>[2x]PAWTTFRVGLFCGIFIVLNITLVLAAVFKLETDRSIWPLIRIYRGGFLLIEFLFLLGINTYGWRQAGVNHVLIFELNPRSNLSHQHLFEIAGFLGILWCLSLLACFFAPISVIPTYVYPLALYGFMVFFLINPTKTFYYKSRFWLLKLLFRVFTAPFHKVGFADFWLADQLNSLSVILMDLEYMICFYSLELKW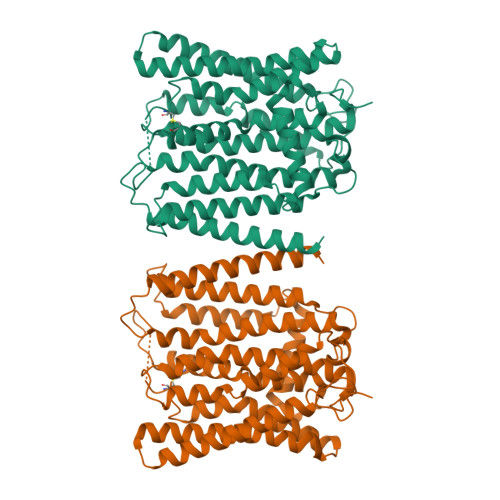DESKGLLPNNSEESGICHKYTYGVRAIVQCIPAWLRFIQCLRRYRDTKRAFPHLVNAGKYSTTFFMVTFAALYSTHKERGHSDTMVFFYLWIVFYIISSCYTLIWDLKMDWGLFDKNAGENTFLREEIVYPQKAYYYCAIIEDVILLFAWTIQISITSTTLLPHSGDIIATVFAPLEVFRRFVWNFFRLENEHLNNCGEFRA>[2x]MKVVLSLGGSVLSNESEKIREFAKTIESVAQQNQVFVVVGGGKLAREYIKSARELGASETFCDYIGIAATRLNAMLLISAIP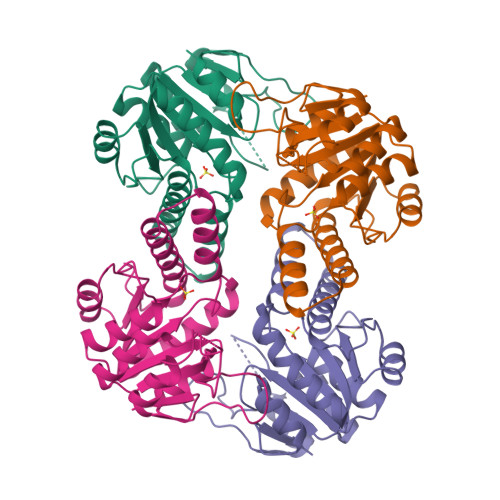SAAKKVPVDFMEAEELSKLYRVVVMGGTFPGHTTDATAALLAEFIKADVFINATNVDGVYSADPKSDTSAVKYDRLSPQQLVEIVSRSSAKAGTNVVIDLLAAKIIERSKIKTYVILGTPENIMKAVKGEAVGTVIA> VQAVAVLKGDAGVSGVVKFEQASESEPTTVSYEIAGNSPNAERGFHIHEFGDATNGCVSAGPHFNPFKKTHGAPTDEVR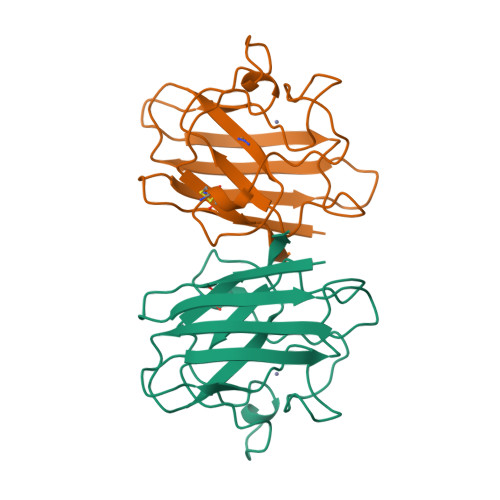HVGDMGNVKTDENGVAKGSFKDSLIKLIGPTSVVGRSVVIHAGQDDLGKGDTEESLKTGNAGPRPACGVIGLTN> XADVAGTSNRDFRGREQRLFNSEQYNYNNSLNGEVSVWVYAYYSDGSVLVINKNSQYKVGISETFKALKEYREGQHNDSYDEYEVNQSIYYPNGGDARKFHSNAKPRAIQIIFSPSVNVRTIKMAKGNAVSVPDEYLQRSHPWEATGIKYRKIKRDGEIVGYSHYFELPHEYNSISLAVSGVHKNPSSYNVGHNVMDVFQSCDLALRFCNRYWAE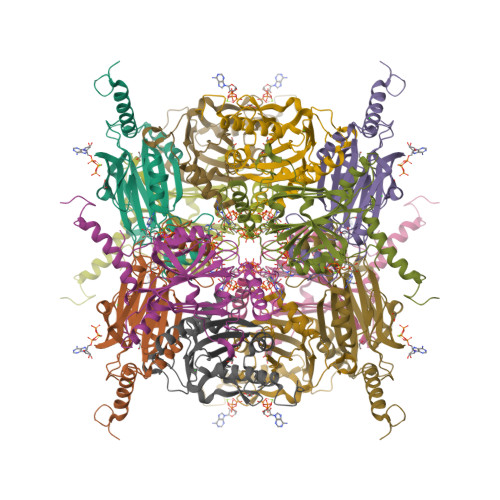LELVNHYISPNAYPYLDINNHSYGVALSNRQ>MGAHSKEMAPLMGKRTTAPGGNPVVLTEKRPADLTPTKKSAHFFLEIEGFEPNPTVTKTSPPIFSKPMDSNIRQCLSGNCDDMDSPQSPQDDVTETPSNPNSPSANLAKEEQRQKKKRLKKRIFAAVSEGCVEELRELLQDLQDLCRRRRGLDVPDFLMHKLTASDTGKTCLMKALLNINPNTKEIVRILLAFAEENDILDRFINAEYTEEAYEGQTALNIAIERRQGDITAVLIAAGADVNAHAKGVFFNPKYQHEGFYFGETPLALAACTNQPEIVQLLMENEQTDITSQDSRGNNILHALVTVAEDFKTQNDFVKRMYDMILLRSGNWELETMRNNDGLTPLQLAAKMGKAEILKYILSREIKEKPLRSLSRKFTDWAYGPVSSSLYDLTNVDTTTDNSVLEIIVYNTNIDNRHEMLTLEPLHTLLHTKWKKFAKYMFFLSFCFYFFYNITLTLVSYYRPREDEDLPHPLALTHKMSWLQLLGRMFVLIWATCISVKEGIAIFLLRPSDLQSILSDAWFHFVFFVQAVLVILSVFLYLFAYKEYLACLVLAMALGWANMLAYTRGFQSMGMYSVMIQKVILHDVLKFLFVYILFLLGFGVALASLIEKCSKDKKDCSSYGSFSDA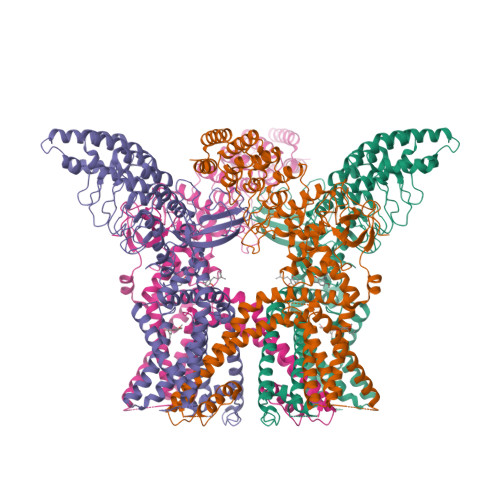VLELFKLTIGLGDLNIQQNSTYPILFLFLLITYVILTFVLLLNMLIALMGETVENVSKESERIWRLQRARTILEFEKMLPEWLRSRFRMGELCKVADEDFRLCLRINEVKWTEWKTHVSFLNEDPGPIRRTADLNKIQDSSRSNSKTTLYAFDELDEFPETSVLVPRGSAAAWSHPQFEK[4x]> MYERFTDRARRVVVLAQEEARMLNHNYIGTEHILLGLIHEGEGVAAKSLESLGISLEGVRSQVEEIIGQGQQAPSGHIPFTPRAKKVLELSLREALQLGHNYIGTEHILLGLIREGE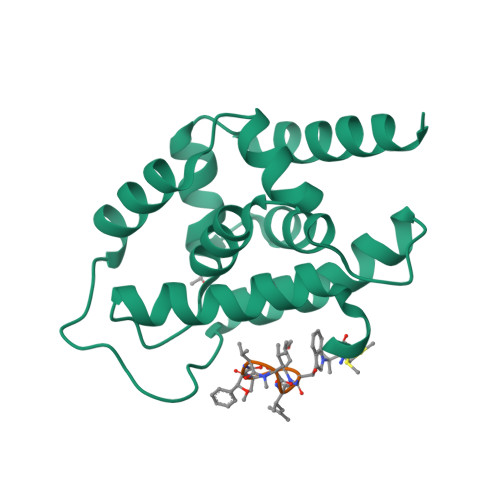GVAAQVLVKLGAELTRVRQQVIQLLSGYLEHHHHHH;> WLAFVLV>MRHEAPMQMASAQDARYGQKDSSDQNFDYMFKLLIIGNSSVGKTSFLFRYADDSFTSAFVSTVGIDFKVKTVFKNEKRIKLQIWDTAGQERYRTITTAYYRGAMGFILMYDITNEESFNAVQDWSTQIKTYSWDNAQVILVGNKCDMEDERVISTERGQHLGEQLGF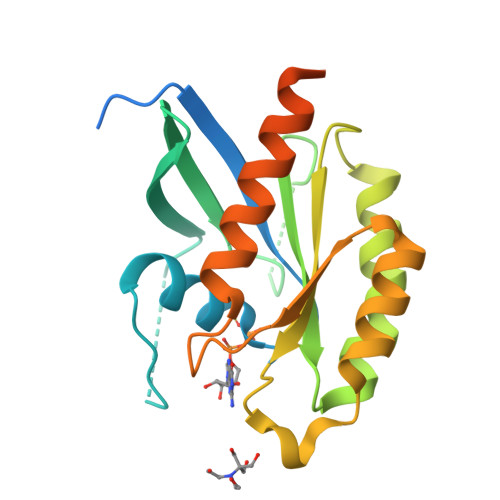EFFETSAKDNINVKQTFERLVDIICDKMSESLETDPAITAAKQNTRLKETPPPPQPNCAC[2x]> VHQVLYRALVSTKWLAESVRAGKVGPGLRVLDASWYSPGTREARKEYLERHVPGASFFDIEECRDKASPYEVMLPSEAGFADYVGSLGISNDTHVVVYDGDDLGSFYAPRVWWMFRVFGHRTVSVLNGGFRNWLKEGHPVTSEPSRPEPAIFKATLNRSLLKTYEQVLENLESKRFQLVDSRAQGRYLGTQPEPDAVGLDSGHIRGSVNMPFMNFLTEDGFEKSPE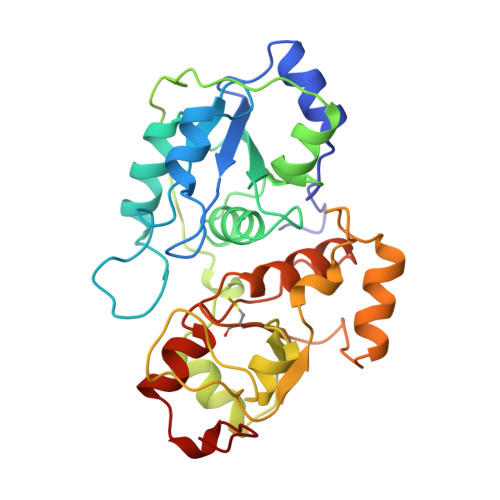ELRAMFEAKKVDLTKPLIATCRKGVTACHIALAAYLCGKPDVAIYDGSWFEWFHRAPPETWVSQGKGGKA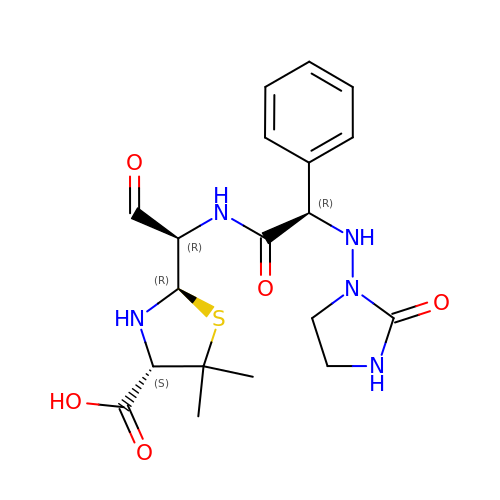(2R,4S)-5,5-dimethyl-2-[(1R)-2-oxo-1-({(2R)-2-[(2-oxoimidazolidin-1-yl)amino]-2-phenylacetyl}amino)ethyl]-1,3-thiazolidine-4-carboxylic acid | C19 H25 N5 O5 S | RSQZNYWGVGFVHY-HGTKMLMNSA-N> MPHDPGATRLLAISPHLDDAVLSFGAGLAQAAQDGANVLVYTVFAGAAQPPYSPAAQRMHTIWGLAPDDDAVLYRRKEDIAALDHLRVAHRHGRFLDSIYRKLPDGRWLTAHVEGRQKLAVNDHSPDSDHDLVGEVADDIRSIIDEFDPTLVVTCAAIGEHPDHEATRDAALFATHEKNVPVRLWEDLPYAVFKSGAVELPQGFRLG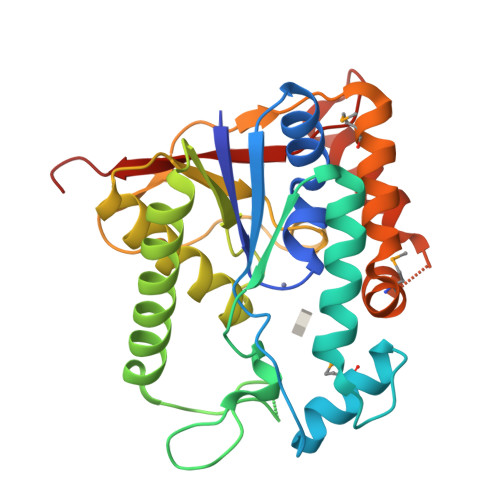SADVSSVKPEMRSQKFQAVERYSSQMVLLNGSENNLFDRLDEHARQNAPHGGYGETTWPVVRSDDS>G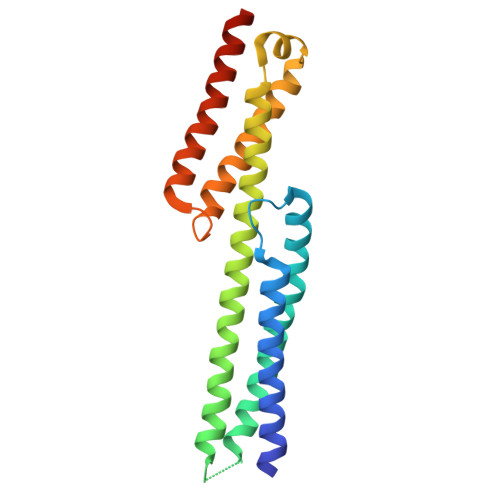SHMAYAQFFSDVREAEGQLQKLQEALRRKYSCDRSATVTRLEDLLQDAQDEKEQLNEYKGHLSGLAKRAKAVGSGSGNQEAQEAVTRLEAQHQALVTLWHQLHVDMKSLLAWQSLRRDVQLIRSWSLATFRTLKPEEQRQALHSLELHYQAFLRDSQDAGGFGPEDRLMAEREYGSCSHHYQQLLQSLEQGAQEE[2x]Omega transaminases (ω-TAs) can mediate the chiral amination of several unnatural substrates without the requirement of an α-COOH group and are highly relevant in the production of several pharmaceutical intermediates of commercial interest. In this work, we successfully overexpressed and characterized the two recombinant transaminases TA_2799 and TA_5182 from P. putida KT2440 and solved their crystal structures. The overall structural fold of the TA_5182 and TA_2799 enzymes is similar to that observed for other class III fold type I TAs with two α/β domains. There are two highly flexible loops present in the structures of TA_2799 and TA_5182 that mediate the entry and exit of the cofactor and the substrate/byproduct into the active site of the enzyme, leading to significant conformational changes in the enzyme structure.

The crystal structure of TA_2799 was determined at a resolution of 1.76 Å in the PLP-bound holo form. The PLP-bound state of TA_2799 is similar to most of the structures found in the PDB, which is the catalytically competent state of the enzyme. Continuous high-quality electron density could be seen for the covalently bound internal aldimine form of the PLP bound to the catalytic K286 residue in both the subunits. The PLP molecule is linked to the ε-NH2 group of the catalytic K286 via a covalent Schiff base, and the pyrimidine ring of the cofactor molecule is sandwiched between the Y150 and I259 residues. The protonated pyrimidine nitrogen is stabilized by hydrogen bonded interactions with D257, and the hydroxyl group of the ring forms a water mediated hydrogen bond with E224. The phosphate group of PLP is stabilized by an intricate hydrogen bonding network, either directly or via water molecules, to S118, S285, Y150, and T323ʹ similar to the “phosphate group binding cup (PGBC)” described by Denesyuk et al.. On the other hand, the L322 position in TA_2799 is usually occupied by an aromatic amino acid. In TA_2799, the side chain of L322 is not bulky enough to cause this change, and as a result, the phosphate group of PLP may not be as tightly coordinated when the PLP molecule is bound to the enzyme. In TA_2799, C324 occupies the same position. C324 is not adequate to cover the crater, so the crater in the crystal structure of TA_2799 is filled with solvent molecules instead.

>[2x]MSTHSSTVQNDLAALIHPNTNLAQHREVGPLVIARGDGVRVFDEQGNAYIEAMSGLWSAALGFSEQRLVDAAVEQFKQLPYYHSFSHKTNAPAAALAAKLAALAPGDLNHVFFTNSGSEANDSVVKMVWYVNNALGRPAKKKFISRQQAYHGATVAAASLTGIPSMHRDFDLPAIPVHHLTCPNFYRFARPGESQEAFTVRLANELERYILAEGPETIAAFIGEPVIAAGGVIPPPTGYWAAIQAVCKRYDILVVIDEIITGFGRLGTMFGSQLYGIQPDIMVLSKQLTSSYQPLAAVVVSDAMNDVLVSQSQRLGAFAHGLTCTGHPVATAVALENIRIIEERDLVGHVQHLAPVFQRHLRAFEDHPLVGNVRGVGLMGGIELVADKATRQPFAQPGTLGGYVFKQAHKHGLIIRAIYDTIAFCPPLITTQDDIEAIFSAFERTLADATDWARSQHLL>[2x]MTATEELTFESTSRFAEVDVDGPLKLHYHEAGVGNDQTVVLLHGGG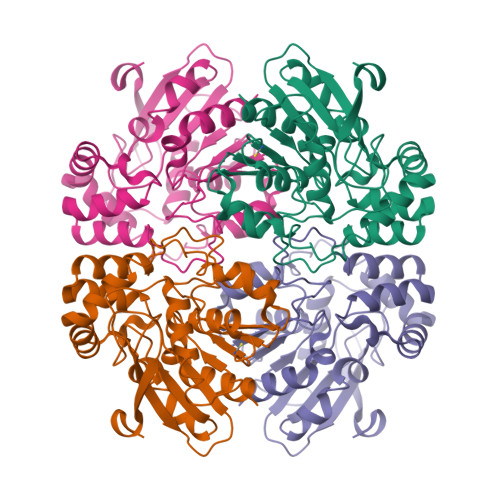PGAASWTNFSRNIAVLARHFHVLAVDQPGYGHSDKRAEHGQFNRYAAMALKGLFDQLGLGRVPLVGNALGGGTAVRFALDYPARAGRLVLMGPGGLSINLFAPDPTEGVKRLSKFSVAPTRENLEAFLRVMVYDKNLITPELVDQRFALASTPESLTATRAMGKSFAGADFEAGMMWREVYRLRQPVLLIWGREDRVNPLDGALVALKTIPRAQLHVFGQCGHWVQVEKFDEFNKLTIEFLGGGR> MRGSGQFRVIGPGHPIRALVGDEAELPCRISPGKNATGMEVGWYRSPFSRVVHLYRNGKDQDAEQAPEYRGRTELLKESIGEGKVALRIQNVRFSDEGG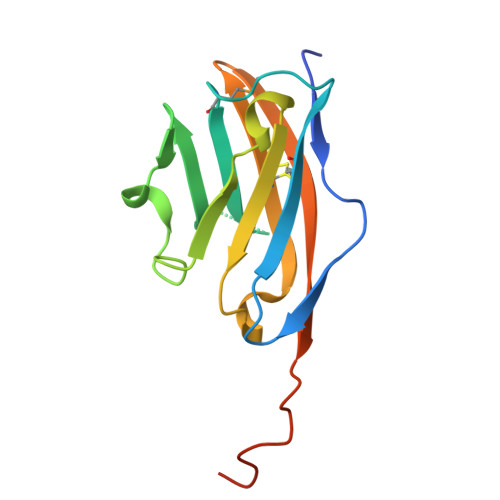YTCFFRDHSYQEEAAVELKVEDPFYWINPGRSRSHHHHHH>[2x]MVNVTVAYQTSAEPAKVAQADNTFAKESGATVDWRKFDSGASI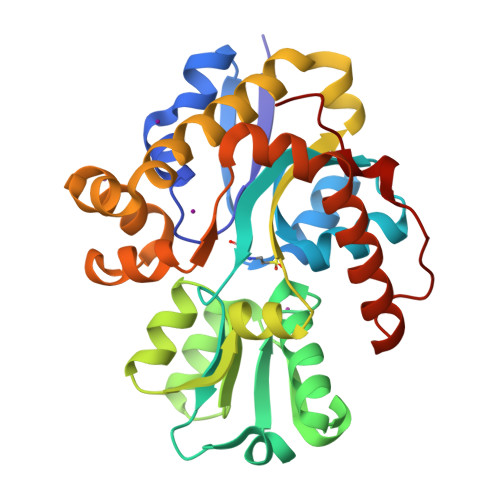VRALASGDVQIGNLGSSPLAVAASQQVPIEVFLLASKLGNSEALVVKKTISKPEDLIGKRIAVPFISTTHYSLLAALKHWGIKPGQVEIVNLQPPAIIAAWQRGDIDGAYVWAPAVNALEKDGKVLTDSEQVGQWGAPTLDVWVVRKDFAEKHPEVVKAFAKSAIDAQQPYIANPDVWLKQPENISKLARLSGVPEGDVPGLVKGNTYLTPQQQTAELTGPVNKAIIDTAQFLKEQGKVPAVANDYSQYVTSRFV> QAQITGRPEWIWLALGTALMGLGTLYFLVKGMGVS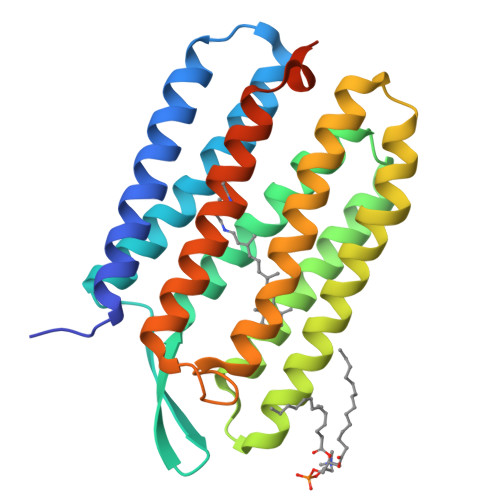DPDAKKFYAITTLVPAIAFTMFLSMLLGYGLTMVPFGGEQNPIYWARYADWLFTTPLLLLDLALLVDADQGTILALVGADGIMIGTGLVGALTKVYSYRFVWWAISTAAMLYILYVLFFGFTSKAESMRPEVASTFKVLRNVTVVLWSAYPVVWLIGSEGAGIVPLNIETLLFMVLDVSAKVGFGLILLRSRAIFGEAEAPEPSAGDGAAATSD> QSACTLQSETHPPLTWQKCSSGGTCTQQTGSVVIDANWRWTHATNSSTNCYDGNTWSSTLCPDNETCAKNCCLDGAAYASTYGVTTSGNSLSIGFVTQSAQKNVGAR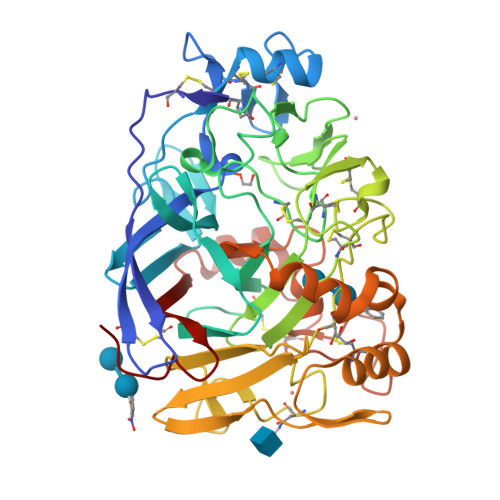LYLMASDTTYQEFTLLGNEFSFDVDVSQLPCGLNGALYFVSMDADGGVSKYPTNTAGAKYGTGYCDSQCPRDLKFINGQANVEGWEPSSNNANTGIGGHGSCCSEMDIWEANSISEALTPHPCTTVGQEICEGDGCGGTYSDNRYGGTCDPDGCDWNPYRLGNTSFYGPGSSFTLDTTKKLTVVTQFETSGAINRYYVQDGVTFQQPNAELGSYSGNELNDDYCTAEEAEFGGSSFSDKGGLTQFKKATSGGMVLVMSLWDDYYANMLWLDSTYPTNETSSTPGAVRGSCSTSSGVPAQVESQSPNAKVTFSNIKFGPIGSTGNPSG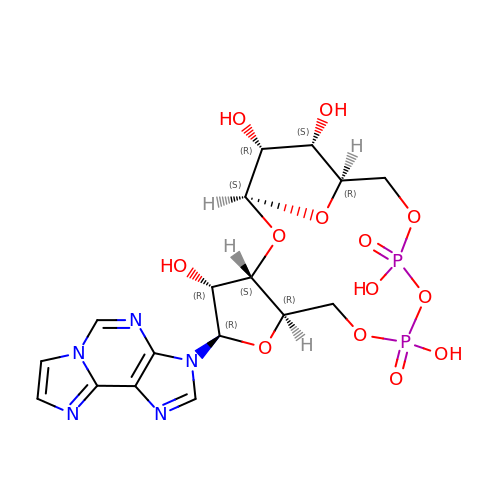(1S,3S,4R,5R,7R,15R,16S,17R)-5-imidazo[2,1-f]purin-3-yl-10,12-bis(oxidanyl)-10,12-bis(oxidanylidene)-2,6,9,11,13,18-hexaoxa-10$l^{5},12$l^{5}-diphosphatricyclo[13.2.1.0^{3,7}]octadecane-4,16,17-triol | C17 H21 N5 O13 P2 | LFJBQYHLOPJAJZ-DLFWLGJNSA-N P-CRESOL | C7 H8 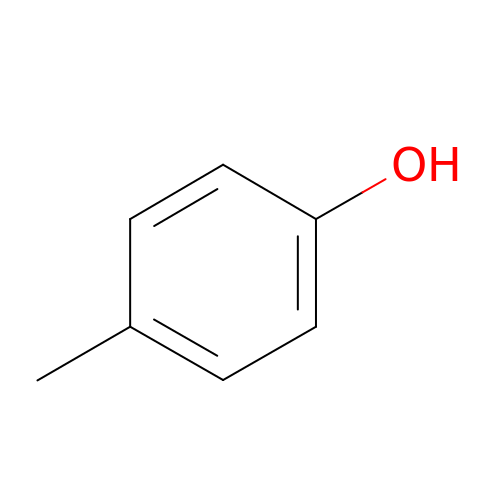O | IWDCLRJOBJJRNH-UHFFFAOYSA-N> MGPVAGNYVHDFTANGTSSSFYTIAGNLSTSKGTATYNGKTLTQCLKMETATSISFTAPSAGKLTLVFAEAAATAKVDGNKVTASNGIITVDLAQGAHTITKADACNLFYMEYAAL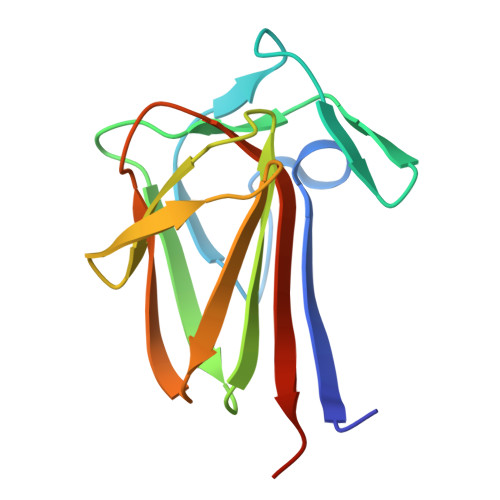EHHHHHH>MAAQNGKDLLIKLDLTGSGQFETIAGLRATRISFNAETVDVTSLESQGGWRELLGGAGVRSASISGAGVFKDADTDERARQIFFDGEVPEFQVIIPDFGIVQGPFMITSIDYAGSHNGEASYELAMASAGALSFTAI[2x];>MAFHEVRFPANLSFGSVGGPERRTEIVTLSSGHEERNSPWAHSRRHYDAGVGLRSLDDVERLIAFFEARGGQLHGFRWKDWADFKSCPASRAVAHEDQLIGMGDGVTTAFQLVKTYVSGGQSYLRPIVKPVEGTVKLGIAGDHQAEAVNFAVDHATGIVSFN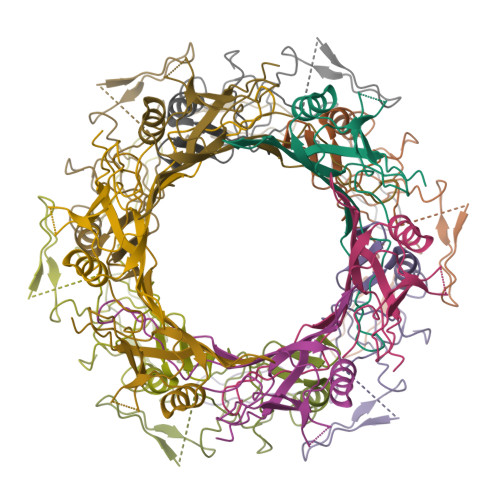EPPPQGARVTAGFEFDVPVRFDTDRIAVSVQSFQAGDLPQVPVVEVRI[2x]> QDNSRYTHFLTQHYDAKPQGRDDRYCESIMRRRGLTSPCIDINTFIHGNKRSIKAICENKNGNPHRENLRISKSSFQVTTCKLHGGSPWPPCQYRATAGFRNVVVACENGLPV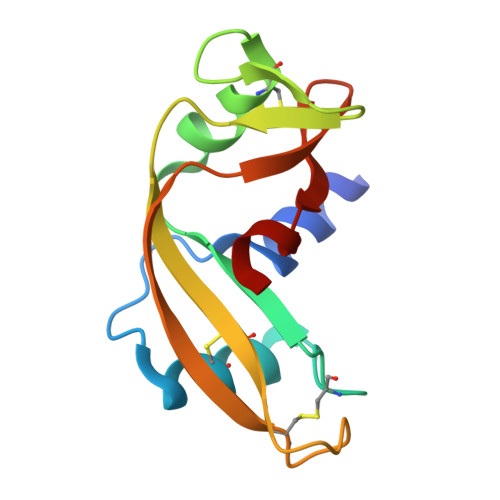HLDQSIFRRP>[4x]ADTIVAVELDTYPNTDIGDPSYP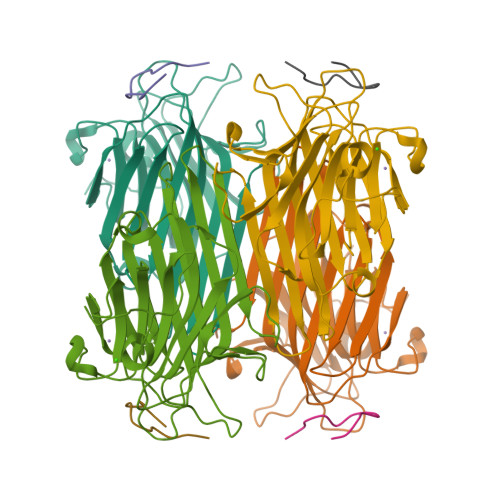HIGIDIKSVRSKKTAKWNMQNGKVGTAHIIYNSVDKRLSAVVSYPNADSATVSYDVDLDNVLPEWVRVGLSASTGLYKETNTILSWSFTSKLKSNSTHETNALHFMFNQFSKDQKDLILQGDATTGTDGNLELTRVSSNGSPQGSSVGRALFYAPVHIWESSAVVASFEATFTFLIKSPDSHPADGIAFFISNIDSSIPSGSTGRLLGLFPDAN;>DVFYPYPYASGS[4x]>MKPKVVLTHWVHPEIIELLSASADVIPNTTRETLPRSEVIARAKDADALMAFMPDSIDSAFLEECPKLRVIGAALKGYDNFDVNACTRHGVWLTIVPDLLTIPTAELTIGLLLGLTRHMLEGDRQIRSGHFQGWRPTLYGSGLTGKTLGIRGMGAVGRAIAQRLAGFEMNLLYCDEIPLNAEQEKAWHVQRVTLDELLEKCDYVVPMVPMAAETLHLIDATALAKMKTGSYLINACRGSVVDENAVIAALASGKLAGYAADVFEMEEWIRADRPQA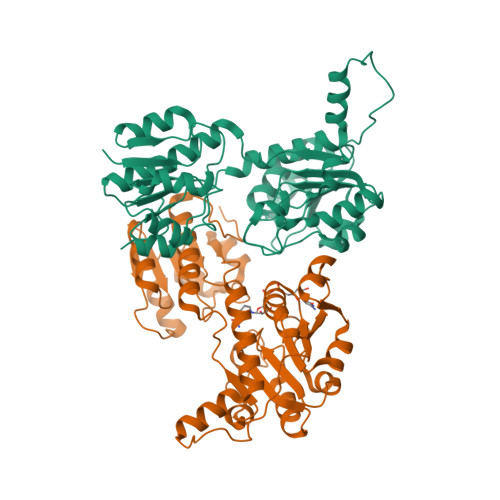IPKALLDNTAQTFFTPHLGSAVKEVRLEIERQAAMNIIQALAGEKPMGAINQPYPGVKAALE[2x]> MRRNTFIKKMSVLLCCQALSLSLFAQQQKVDTAHIYSIPEIMVSDPYQTREVRSASPLQVFNKEELKNLQALQVSDAVKHFAGVTVKDYGGIGGLKTVSIRSLGAQHTAVSYDGITVSDCQTGQVDIGRFSLNNVDRLSLNNGQSDNIFQPARFFASAGILNIQTLTPHFKEDKPTNIAAEFKTGSWGLVNPSLFLEQQLNKKWSMTANGEWMSSDGHYPFTLRYGNDADVQVSKEKRRNTDVENLRAEISAFANLSDKEQWRLKAYYYQSSRGLPNATTLYYDFSRQNLRDKNTFIQSQYKKEFSRKWVFQTSAKWNWSYQNYQDPDALTSVGGTDNSYYQQEYYLSASALYRIWNNLSFSLSTDGSINTMNANLQNFVSPTRYSWLTAFAGKYVNEWVTLSASALATVINEKAKNGGNAGNHRKLSPNVSISLKPFHNEELRFRFFYKDIFRLPSFNDLYYDKAGNINLKPESATQYNIGITYSKAINNFIPYLSATVDAYHNKVTDKIVATPTKNLFIWSMVNLGKVDIKGIDATASLSLQPLDKLRINLSGNYTYQRALDVTNSNPNSPEGKVYKHQIAYTPRVSASGQAGIETPWLNLSYSFLFSGKRYMLGQNISDNRLDSYSDHSISAYRDFKIQKVTASLNLEVLNLMNRNYEIVKNFPMPGRSVRVTIGVRYGGGHHHHHH;> MQKGLLYNMLLRLGKYFFLFPLFFIACDDLEDKPSIVPESNGDVFETGTAEMYILSEGLFNQNNSSLARYSFNRQRCTNNYFSANNQRGLGDTANDIAIYGNKIYVVVNVSSTVEVIDFPTGKSIRQISMLRDNGSSRQPRAIAFDKDKAYICSYDGTVARIDTTSLEIEEIVTVGRNAEDICVQNGKLYVSNSGGLDYSGPGVDTTVSVIDITTFKETKKIEVGPNPGKILPGLEEAVYVVTRGTDIEAGDYHLVKIDSRTDAVAITYDEKVLSFAIDGPIAYLYTYDYQTKDSAIKVFDLNAGTVIRDNFITDGTAIQTPFSIQLNPFSGNIYITEAYNYTVKGDVLCFNQQGQLQYRLNDIGLNPNTVVFSDKASQNEAGDTPEDPNAPSAFANKVFEYIPAPGQFINTTTSAYEDGFSAGQVLEHATEKLKKKSVISLGGFGGTITVGFHQSIRNSKGEYDFRILGNASYNQNTGTGALGGSAEPGIVLVSKDENGNGLPDDEWYELAGSEYGKDTETRNYEITYYRPQPANGDVRWTDNQGGEGFVYRNSYHQQDSYYPNWIEEDEITFRGTRLKDNAINEGGTWVGYCYPWGYADNHPNRSEFSQFKIDWAVDQNGNHVELDKIDFVKIYTAVNQNVGWMGEISTEVMTVEDLHFEN

Contrasting with Enterobacteria, members of the dominant genus Bacteroides often encode several BtuB vitamin B12 outer membrane transporters together with a conserved array of surface-exposed B12-binding lipoproteins. Here we show that the BtuB transporters from Bacteroides thetaiotaomicron form stable, pedal bin-like complexes with surface-exposed BtuG lipoprotein lids, which bind B12 with high affinities. Closing of the BtuG lid following B12 capture causes destabilisation of the bound B12 by a conserved BtuB extracellular loop, causing translocation of the vitamin to BtuB and subsequent transport. We propose that TonB-dependent, lipoprotein-assisted small molecule uptake is a general feature of Bacteroides spp. that is important for the success of this genus in colonising the human gut.

To obtain more experimental insight into the dynamics of BtuG lid opening, we determined the structure of the BtuB1G1 (i.e. the BtuBG complex of locus 1) complex by cryo-EM. BtuG1 is ~70 kDa in size due to the presence of a C-terminal extension of ~250 residues that is homologous to the BtuH2 protein that was recently shown to bind B12 on the cell surface of B. theta; thus, BtuG1 contains two B12 binding sites. The additional BtuH domain increases the size of the extra-membrane part of the complex substantially, facilitating structure determination by cryo-EM. We obtained ~3.2 Å maps for the complex in the absence of CNCbl. The additional BtuH domain (BtuG1 H-domain) is clearly visible and appears to be docked to BtuG1, in a position that would not allow B12 binding. The resolution of the BtuG1 H-domain was substantially worse than the rest of the complex, implying some degree of conformational flexibility. Interestingly, and contrasting with substrate-free structures of SusCD glycan transporters, the BtuB1G1 EM structure is very similar to the BtuB2G2 crystal structure with a closed BtuG lid, and there are no particle populations with open BtuG1 lids. We also collected data for BtuB1G1 in the presence of 2 molar equivalents CNCbl, but analysis of the dataset suggested a destabilising effect on the DDM-solubilised complex caused by the presence of CNCbl, analogous to BtuB2G2.> TESGTAAQDPEALAA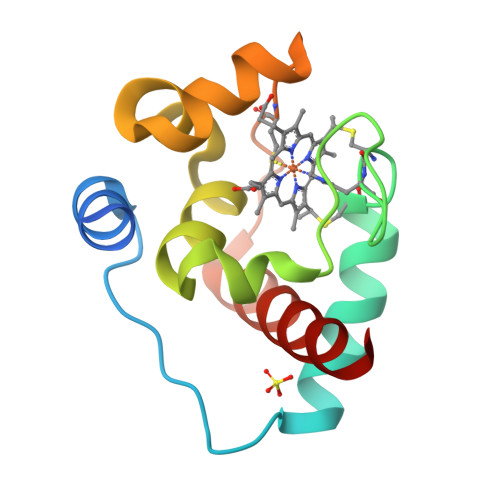EIGPVKQVSLGEQIDAALAQQGEQLFNTYCTACHRLDERFIGPALRDVTKRRGPVYIMNVMLNPNGMIQRHPVMKQLVQEYGTMMTDMALSEEQARAILEYLRQVAENQ>GPHMPTEVILRGYRNAQHQYAAINHYEQIAGRICEDYPREPPVESRRYKSELRDPAFTHRR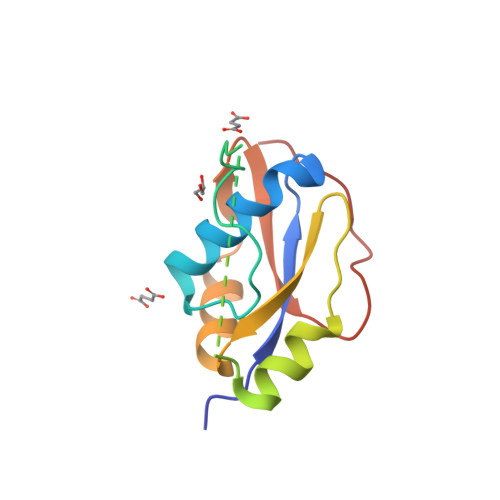ALTPEERAKVNRAMSGEHWVKVTFESAEAADKAVYSSPQLIQGHLVYAEYYKGVPPAQDEAIPD[4x]> SMLRAQATGNIGVLVSRVTNPFFAGLFDAIERELHAHGYQVMITQTYDDPEAEERFLKQLKSRELDGV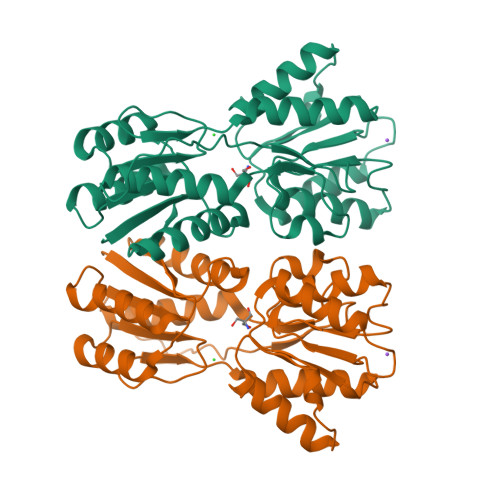ILASVEAPDRVMAVAKAFPGRVVVVNADVQIPGATSLVLPHYQATRDALDYLFNQGHRRFAYVSGGTISGAHHGQSRTQAFLDFMQAHQLLVAQDLLFGQIHTAKEGQAVGKQLASLAPNVRPDAVFTNSDEVAVGVIDSLLAADVKVPDDIAVMGYDDQPFAPFAKIPLTTVHQPVASMAAAATHELLKGLGRQVAQDTQPTLHLSLKIRQSA> AE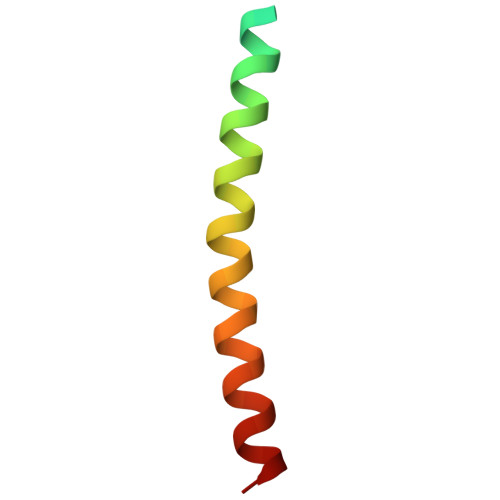GDDPAKAAFDSLQASATEMIGYAWAMVVVIVGATIGIKLFKKFTSKAS>MRVLVSNDDGVDAPGIKILADALRNAGHEVMVVAPDRDRSGASNSLTLDTPIRAKQIDMHTYSVAGTPTDCVHLALTGLLNYDPDIVVSGINNTGNLGDDVIYSGTVSAAMEGRFLGLPAVAVSLVTLYREGQQAPQYETAAHAAINIVAQLKTDPLPADTILNVNVPDVTWQQMRGFKVTRLGNRHRSAPCLTQTDPRGHTIYWIGPAGPEQDAGPGTDFDAVRNTYISITPIHVDLTRYQALENVTRWTDRL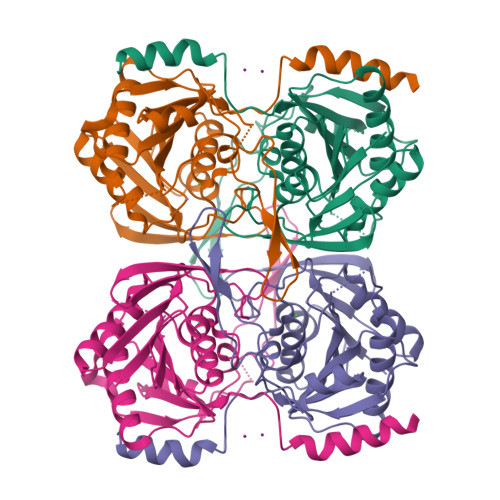TAHMDWPTLEHHHHHH[2x]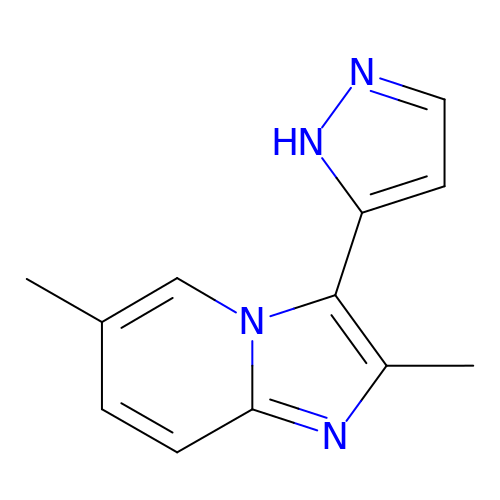2,6-dimethyl-3-(1H-pyrazol-5-yl)imidazo[1,2-a]pyridine | C12 H12 N4 | FLABUTFVIDAMFH-UHFFFAOYSA-N> TGCGC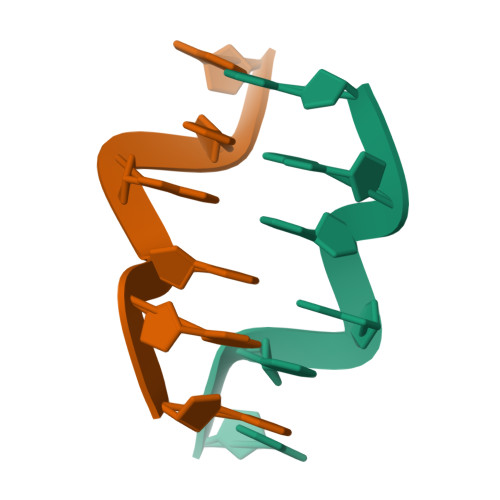G;> CGCGCA;>[2x]TG>[6x]MQKLIMGNWKMNGNSTSIKELCSGISQVQYDTSRVAIAVFPSSVYVKEVISQLPEKVGVGLQNITFYDDGAYTGEISARMLEDIGCDYLLIGHSERRSLFAESDEDVFKKLNKIIDTTITPVVCIGESLDDRQSGKLKQVLATQLSLILENLSVEQLAKVVIAYEPVWAIGTGVVASLEQIQETHQFIRSLLA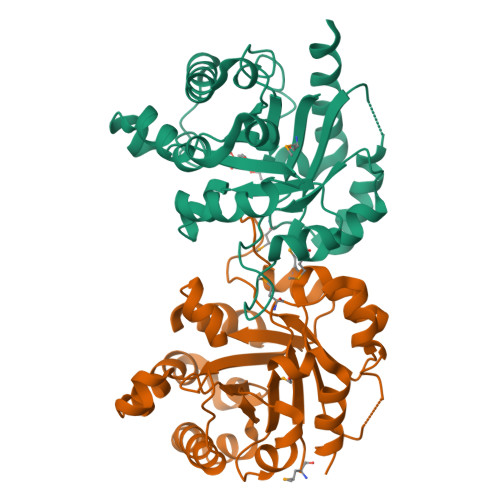KVDERLAKNIKIVYGGSLKAENAKDILSLPDVDGGLIGGASLKAAEFNEIINQANKICTE Enteroviruses (EV), an important genus of this family, include a variety of human pathogens, such as polioviruses and the human enterovirus D68 (EV-D68). EV-D68 is a causative agent of childhood respiratory infections and occasionally leads to neurological diseases. The capsid of EVs consist of 60 copies of each of the viral proteins VP1, VP2 and VP3, that form an icosahedral shell with pseudo T=3 symmetry, and 60 copies of VP4 that form a network on the interior surface of the capsid. In summary, the structural and functional analyses showed that sialic acid is a functional cellular receptor for EV-D68.

The crystal structures were determined of EV-D68 when in complex with 3′SLN, 6′SL or 6′SLN. All three receptor analogues were observed to bind near the ‘eastern end' of the canyon. In all three structures the Neu5Ac moiety is well accommodated in a wide crater formed by VP1 and VP3 within the same protomer6. The contact region for all three receptor analogues is the VP1 C terminus, VP3 C terminus and VP3 CD loop. In contrast, 6′SLN (as also 6′SL) adopts a bent conformation such that the GlcNAc moiety, which is furthest away from the Neu5Ac moiety, is well clear of the virus surface which, therefore, permits the presence of BSA. The same conformational changes occurred in each of the three complexes. Thus binding of sialylated receptor analogues onto EV-D68 causes a partial collapse of the pocket, leading to the displacement of the pocket factor. However, in these sialylated receptor analogue bound structures, the VP4 density is still present and the particle size is not altered, indicating that sialylated glycan binding of EV-D68 at room temperature represents an initial event of the viral entry process. Thus, binding of the sialylated receptor analogues displaces the pocket factor through long range structural rearrangements of the virus. In summary, binding of sialic acid receptor analogues to EV-D68 ejects the pocket factor and therefore presumably destabilizes the virus to facilitate viral uncoating.

> VESIIKTATDTVKSEINAELGVVPSLNAVETGATSNTEPEEAIQTRTVINQHGVSETLVENFLGRAALVSKKSFEYKNHASSSAGTHKNFFKWTINTKSFVQLRRKLELFTYLRFDAEITILTTVAVNGNNDSTYMGLPDLTLQAMFVPTGALTPKEQDSFHWQSGSNASVFFKISDPPARMTIPFMCINSAYSVFYDGFAGFEKNGLYGINPADTIGNLCVRIVNEHQPVGFTVTVRVYMKPKHIKAWAPRPPRTMPYMSIANANYKGRDTAPNTLNAIIGNRASVTTMPHNIVTT;> SPSAEACGYSDRVLQLKLGNSAIVTQEAANYCCAYGEWPNYLPDHEAVAIDKPTQPETSTDRFYTLRSVKWESNSTGWWWKLPDALNNIGMFGQNVQYHYLYRSGFLIHVQCNATKFHQGALLVVAIPEHQRGAHDTTTSPGFNDIMKGERGGTFNHPYVLDDGTSIACATIFPHQWINLRTNNSATIVLPWMNVAPMDFPLRHNQWTLAVIPVVPLGTRTMSSVVPITVSIAPMCCEFNGLRHAITQ;> GVPTYLLPGSGQFLTTDDHSSAPVLPCFNPTPEMHIPGQIRNMLEMIQVESMMEINNTDGANGMERLRVDISVQADLDQLLFNIPLDIQLDGPLRNTLVGNISRYYTHWSGSLEMTFMFCGSFMATGKLILCYTPPGGSCPTTRETAMLGTHIVWDFGLQSSITLIIPWISGSHYRMFNSDAKSTNANVGYVTCFMQTNLIVPSESSDTCSLIGFIAAKDDFSLRLMRDSPDIGQSNHLHGAEAAYQ;> GAQVTRQQTGTHENANIATNGSHITYNQINFYKDSYAASASKQDFSQDPSKFTEPVVEGLKAGAPVLK>[4x]HHHHHHSKKPRQKRTATKAYNVTQAFGRRGPE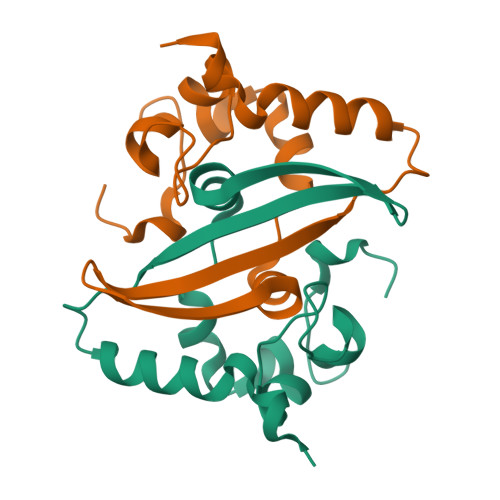QTQGNFGDQELIRQGTDYKHWPQIAQFAPSASAFFGMSRIGMEVTPSGTWLTYTGAIKLDDKDPNFKDQVILLNKHIDAYKTFP>[2x]SVTIDHTTENAAPAQAPVSDRAWALFRALDGKGLVPDGYVEGWKKTFEEDFSPRRGAELVARAWTDPEFRQLLLTDGTAAVAQYGYLGPQGEYIVAVEDTPTLKNVIVCSLCSCTAWPILGLPPTWYKSFEYRARVVREPRKVLSEMGTEIASDIEIRVYDTTAETRYMVLPQRPAGTEGWSQEQLQEIVTKDCLIGVAIPQVPTV;>MDGVHDLAGVQGFGKVPHTVNADIGPTFHA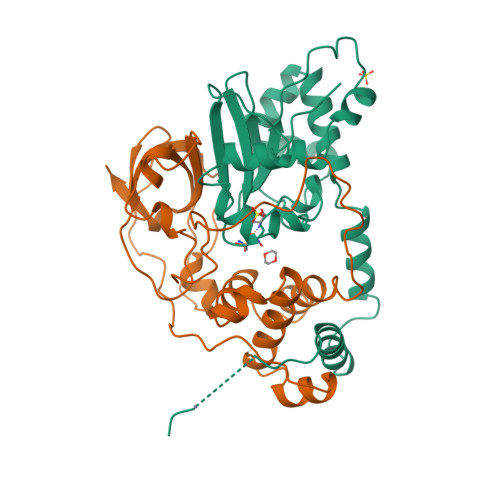EWEHLPYSLMFAGVAELGAFSVDEVRYVVERMEPRHYMMTPYYERYVIGVATLMVEKGILTQDELESLAGGPFPLSRPSESEGRPAPVETTTFEVGQRVRVRDEYVPGHIRMPAYCRGRVGTISHRTTEKWPFPDAIGHGRNDAGEEPTYHVKFAAEELFGSDTDGGSVVVDLFEGYLEPAA[2x]> MSKGFTLEKNLPHQKAGVDAVMNVFVSATPHLTDNVAVRLLANPELKLSEQQYYNNIKNVQAFNGIAHSKDNHNAKSNIIDVSMETGTGKTYTYIKTIFDLNKSFGINKFIIIVPTLSIKAGTVNFLKSDALKEHFRDDYKRELRTYVVESQKNAGKNTKSYMPQAIHDFVEASNFNKKYIHVLVINSGMINSKSLTDTYDTGLLDNQFNTPVDALRAVKPFIIIDEPHRFPTGKKTWENIEKFNAQYIIRYGATFSEGYKNLVYRLTAVDAFNDDLVKGIDAYIEDIVGDGNANLKFVKSDGKEATFELNENNNKKSFKLAKGESLSKTHSAIHDLTLDALNKSTAVLSNGIELKIGSSINPYSYDQTLADNMMRKAVKEHFKLEKELLTQRPRIKPLTLFFIDDIEGYRDGNDISGSLKTKFEEYVLAEANELLKTEQDAFYKNYLEKTVTNISSVHGGYFSKDNSDKDDKIEQEINEILHDKELLLSLDNPRRFIFSKWTLREGWDNPNVFQICKLRSSGSTTSKLQEVGRGLRLPVNEYMCRVKDRNFTLKYYVDFTEKDFVDSLVKEVNESSFKERVPSKFTQELKEQIMAQYPELSSRALMNELFNDEIIDDNDNFKDSDAYSRLKSKYP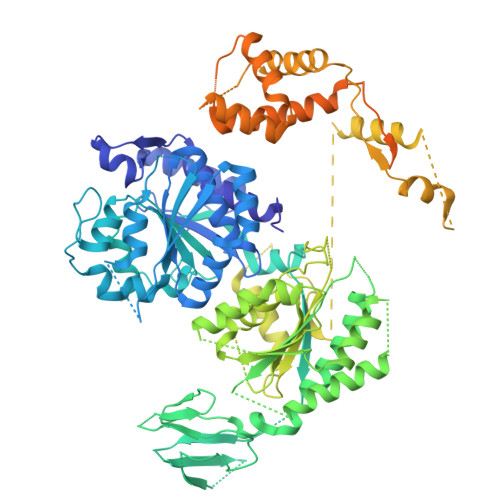AAFPIGVKPGKIKKATDGKRRTKMRVGKFSELKELWDLINQKAVIEYKINSESEFLSIFKSFMLEETERFTKSGVHTRIDKIYIHNDMAMSKSIVSDDDDFAKLNTMSYREFLDNLSQTIFVKHGTLHKVFCDIKDTINITEYLNIQTIRKIKSGFSKYLLNNSFNKFSLGYNLISGSIHPTKFTNADGNPLGEVLSSDLGVLQDNAKAPLDTYLFEEVFYDSELERRNITDREIQSVVVFSKIPKNSIKIPVAGGYTYSPDFAYVVKTAEGDYLNFIIETKNVDSKDSLRLEEKRKIEHAQALFNQISQSVKVEFRTQFANDDIYQLIKSALP>[2x]SKILVFGHQNPDSDAIGSSVAFAYLAKEAWGLDTEAVALGTPNEETAYVLDYFGVQAPRVVESAKAEGVETVILTDHNEFQQSISDIKDVTVYGVVDHHRVANFETANPLYMRLEPVGSASSIVYRMFKENGVSVPKELAGLLLSGLISDTLLLKSPTTHASDIPVAKELAELAGVNLEEYGLEMLKAGTNLSSKTAAELIDIDAKTFELNGEAVRVAQVNTVDINDILARQEEIEVAIQEAIV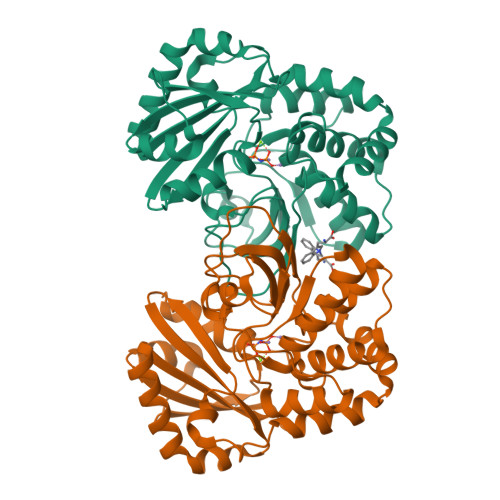TEGYSDFVLMITDIVNSNSEILALGSNMAKVEAAFEFTLENNHAFLAGAVSRKKQVVPQLTESYNA Steviolbioside | C32 H50 O13 | 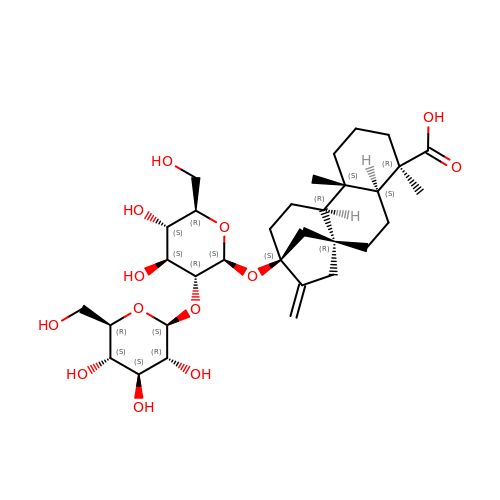OMHUCGDTACNQEX-OSHKXICASA-N> SNPRKFSEKIALQKQRQAEETA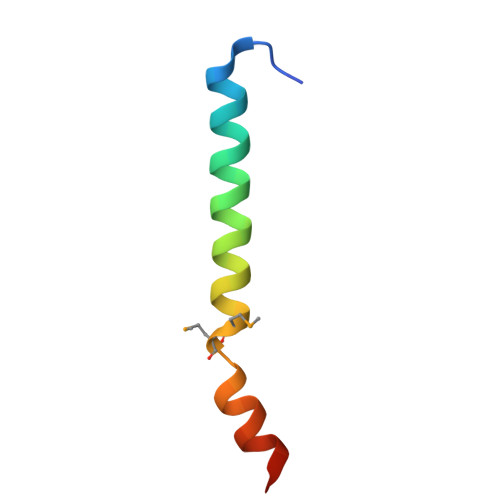AFEEVMMDIGSTRLQAQKLR>MHHHHHHSSGRENLYFQGMNMEITNLKSYKELVTLSAEEKTKDLKDYLNDKNRSESLIKKFKNFYMDLSRQRYSEKTLNKLVEYAEEVELKKKVEKTFMGEKVNMTENRSVLHTALRIPIEKINTHKIIIDNKNVLEDVHGVLKKIEKYSDDIRNGVIKTCKNTKFKNVICIGIGGSYLGTEFVYEAMKYYYYNMELNKNEKDQVNNFNNNYDQDNVFNVRFLANVDPNDVNRAIQNLDQYDTLVIIISKTFTTAETMLNARSIKKWLSLKIKDDENLSKHMVAVSTNLKLTDEFGISRDNVFEFWDWVGGRFSVTSSVGILPLSIAFGYKNMRNFLNGCHDMDEHFLHADLKENIPVLLALTSFYNSHFFDYKNVAILPYFQNLLKFSAHIQQLSMESNGKSVDRNNQPIHYNTCQVYFGEPGTNGQHSFYQLIHQGQVIPVELIGFKHSHFPIKFDKEVVSNHDELMTNFFAQADALAIGKTYEQVKEE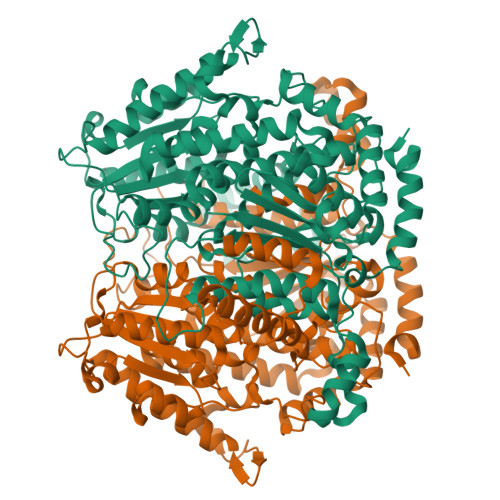NEKNKMSPELLTHKVFNGNRPSTLLLFDELNFYTCGLLLSLYESRIVAEGFLLNINSFDQWGVELGKVLAKEVRNYFNDTRNQKKSDNTYNFNESTKILLNYYLSK[3x]>[4x]SMLKIQAYFNETADLPCQFANSQNQSLSELVVFWQDQENLVLNEVYLGKEKFDSVHSK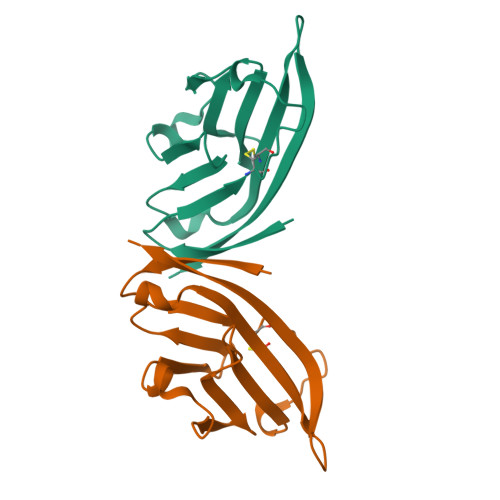YMGRTSFDSDSWTLRLHNLQIKDKGLYQCIIHHKKPTGMIRIHQMNSELSVLA> MKDLKKIESYLDKLRIKEKDGEERKIYAEVLDGRTLKTLYKLSAKGYITAMGGVISTGKEANVFYADGVFDGKPVAMAVKIYRIETSEFDKMDEYLYGDERFDMRRISPKEKVFIWTEKEFRNLERAKEAGVSVPQPYTYMKNVLLMEFIGEDELPAPTLVELGRELKELDVEGIFNDVVENVKR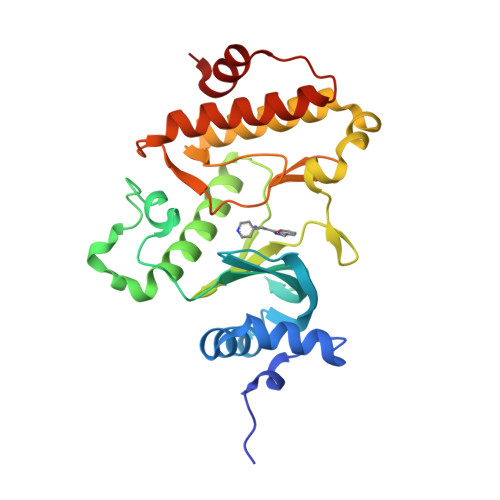LYQEAELVHADLSEYNIMYIDKVYFIDMGQAVTLRHPMAESYLERDVRNIIRFFSKYGVKADFEEMLKEVKGE>MNLIPTVIETTNRGERAYDIYSRLLKDRIIMLGSQIDDNVANSIVSQLLFLQAQDSEKDIYLYINSPGGSVTAGFAIYDTIQHIKPDVQTICIGMAASMGSFLLAAGAKGKRFALPNAEVMIHQPLGGAQGQATEIEIAANHILKTREKLNRILSERTGQSIEKIQKDTDRDNFLTAEEAKEYGLIDEVM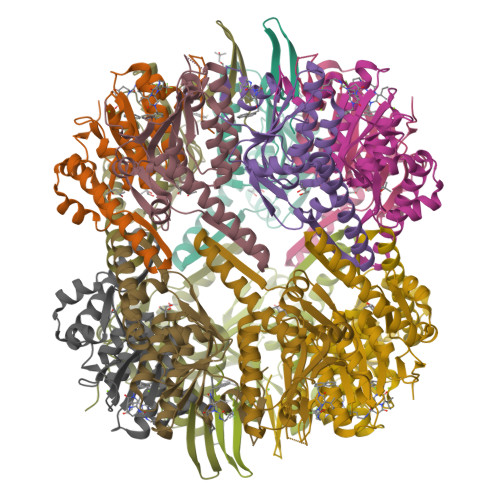VPETK[14x]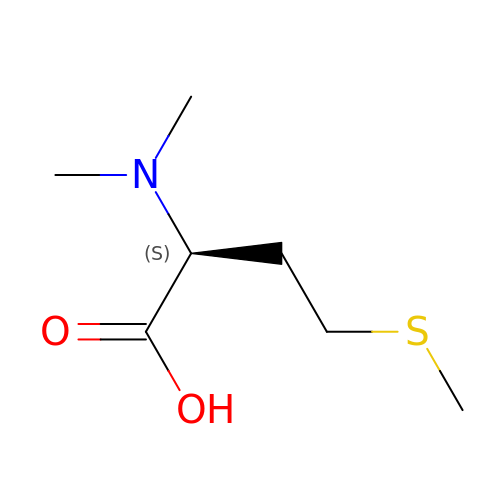N,N-dimethyl-L-methionine | C7 H15 N O2 S | FLEXUHXAXRFRAU-LURJTMIESA-N> MAAPGAGPGPGAPPGLEAALQKLALRRKKVLSAEETELFELAQAAGGAMDPEVFKILVDLLKLNVAPLAVFQMLKSMCAGQRLASEPQDPVAVPLPTTSVPETRGRNRGSSALGGGPALAERSG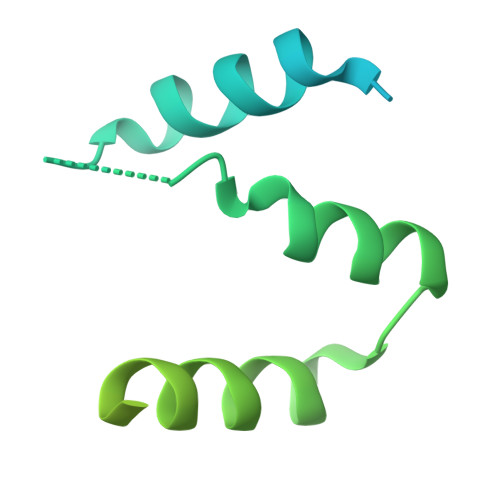REGSSQRMPRQPSATRLPKGGGPGKSPTRST>CGIWALFGSDDCLSVQCLSAMKIAHRGPDAFRFENVNGYTNCCFGFHRLAVVDPLFGMQPIRVKKYPYLWLCYNGEIYNHKKMQQHFEFEYQTKVDGEIILHLYDKGGIEQTICMLDGVFAFVLLDTANKKVFLGRDTYGVIPLFKAMTEDGFLAVCSEAKGLVTLKHSATPFLKVEPFLPGHYEVLDLKPNGKVASVEMVKYHHCRDVPLHALYDNVEKLFPGFEIETVKNNLRILFNNAVKKRLMTDRRIGCLLSGGLDSSLVAATLLKQLKEAQVQYPLQTFAIGMEDSPDLLAARKVADHIGSEHYEVLFNSEEGIQALDEVIFSLETYDITTVRASVGMYLISKYIRKNTDSVVIFSGEGSDELTQGYIYFHKAPSPEKAEEESERLLRELYLFDVLRADRTTAAHGLELRVPFLDHRFSSYYLSLPPEMRIPKNGIEKHLLRETFEDSNLIPKEILWRPKEAFSDGITSVKNSWFKILQEYVEHQVDDAMMANAAQKFPFNTPKTKEGYYYRQVFERHYPGRADWLSHYWMPKWINATDPSARTLTHYKSAVKAAGENLYFQSHHHHHHHHHH[2x]

Here, we use human ASNS, a Class II glutamine-dependent amidotransferase that mediates asparagine biosynthesis, as a model system to evaluate whether EM-derived maps can provide insights into conformational changes that might mediate function in multi-site enzymes. As in all other glutamine-dependent enzymes, catalytic turnover requires that ammonia must move through an intramolecular tunnel connecting the active sites. Human ASNS is also of considerable biomedical interest, having been linked to metastatic progression in breast cancer, sarcoma cell proliferation, and decreased effectiveness of clinical treatments for acute lymphoblastic leukemia. Moreover, ASNS variants are strongly correlated with impaired neural development in children, pointing to the importance of gaining an in-depth understanding of how single residue changes might affect activity by altering the conformational preferences and dynamics of the enzyme.

Arg-142 is conserved in mammalian asparagine synthetases, Sequence and structural alignments, however, show that that cognate residue in Escherichia coli AS-B is isoleucine (Ile-143) even though nearby residues are conserved in both homologs. We were able to determine the structure of the R142I variant dimer at 3.35 Å resolution by cryo-EM in order to assess the validity of these MD simulations. As expected, replacing a polar group by a hydrophobic side chain had little impact on the overall structure of the enzyme (0.483 Å RMSD of WT vs. the R142I variant) although structural changes in the tunnel region are observed that will be the subject of future computational analysis. The N-terminal entrance to the tunnel linking the two active sites is open in the EM structure, similar to that seen in the X-ray structure of the C1A AS-B variant bound to glutamine and AMP. When L-aspartate was varied at saturating levels of L-glutamine, but in the absence of ammonia, the kinetics of PPi formation showed 4- and 2-fold reductions in turnover number for the R142I and R142A variants, respectively. In addition, given that the gate to the tunnel is open in the two variants, as seen in the MD simulations and in the cryo-EM structure of the unliganded R142I variant, ammonia trafficking is expected to be maintained at the WT level and so have little impact on steady-state kinetic properties. Replacing the positively charged Arg-142 side chain by the smaller, hydrophobic side chains of isoleucine or alanine, however, clearly alters how the C-terminal synthetase domain in human ASNS responds to different nitrogen sources. More importantly, these calculations raise the possibility of a role for Arg-142 in maintaining the structural integrity of the tunnel after formation of the β-aspartyl-AMP intermediate; this finding may underpin the observed kinetic properties of the R142I variant although additional experiments and simulations will be needed to support this hypothesis.> MALLEDTSEKVKVYLRIRPFLTSELDRQEDQGCVCIENTETLVLQAPKDSFALKSNERGVGQATHKFTFSQIFGPEVGQVAFFNLTMKEMVKDVLKGQNWLIYTYGVTNSGKTYTIQGTSK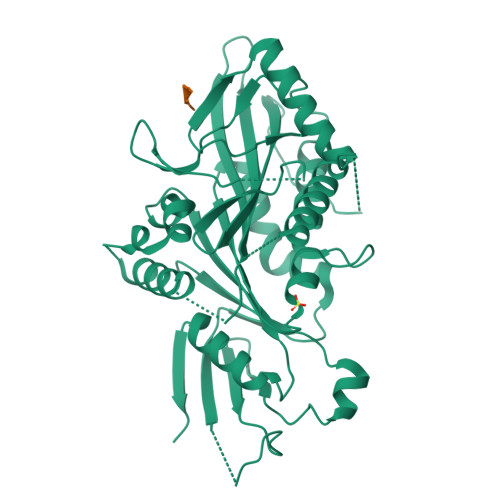DAGILPQSLALIFNSLQGQLHPTPDLKPLLSNEVIWLDSKQIRQEEMKKLSLLIGGLQEEELSTSVKKRVHTESRIGASNSFDSGVAGLSSTSQFTSSSQLDETSQLWAQPDTVPVSVPADIRFSVWISFFEIYNELLYDLLEPPSHQHKRQTLRLCEDQNGNPYVKDLNWIHVRDVEEAWKLLKVGRKNQSFASTHMNQQSSRSHSIFSIRILHLQGEGDIVPKISELSLCDLAGSERCKHQKSGERLKEAGNINTSLHTLGRCIAALRQNQQNRSKQNLIPFRDSKLTRVFQGFFTGRGRSCMIVNVNPCASTYDETLHAAKFSALASQLVHAPLEHHHHHH>[2x]MALTKLVDAGAWQVEVAPAGTVQDSLVFLSPRNFGGVPGTGVDSVAAIEAALAAGDVDLGGEHWFISRPIYCVSGRTIQNGKISTLAAQGSGFMAGSIFAPGNYHPVYVDPVPKLACSSTNGSATITVSSHEFVVGDLVRLSSTRGIIGSDAVLVPWYMQLARVVGVSGDTVKLDAPIDTTETLVVHKATPAGYNARFNKPLFVLERATFRNIEVDTWDYWTADSATFECAFEGIRGKARSVVYGNTFCRTNFDNIDITFSNKASEMAFGSHDTNLSNIKFRADSQNWDSTNSVGISWAESGRRCTLDNWQLLVPQGVNLSVLVRISSHRDVQIRKGFIQVHSSSNNILSVEHYGGDRPPCNNILFEDIDVNATGAAAVVVDVYKSANDSAINAVRFEGISYRGATPSVALMRQRGTTSNQVTGVRASLYSANGGAFLVSSAMAWDVRLYGPGLQVPAAVAVLGRTAVLSASRSNLHALRWVTEAIIGVTSTTPGNVLREAVIPAGTLRASDYIDFVISGSTGGATSTKDVLVGVLDSGSNFQGVGFTAPTTEESYYTVQGRISFPTTGNCLITATIGRAGVGVSYARTLVSISNYTTNDVKLQVQAWVGSSAGSLSVQHGCFAPSELTGKGHHHHHH

Virion-associated depolymerases are large trimeric and multi-domain proteins that constitute the phage arsenal to degrade the polysaccharide layers in their bacterial host. In this study, we elucidated the structural and functional features of the capsular depolymerase KP34gp57 from the Klebsiella phage KP34. The CPS depolymerase KP34gp57 is a large enzyme with a trimeric organization consisting of 630 amino acid residues per chain and an MW of the trimer of ~200 kDa. In this work, we focused on the structure and function of the CPS depolymerase KP34gp57 derived from Klebsiella phage KP34, which efficiently causes a visible halo zone on bacterial lawns of the K63 serotype of K. pneumoniae.

Surprisingly, we collected diffraction data at 2.0 Å resolution, which produced a unit cell and space group (a = 38.3, b = 141.0, c = 81.9; β = 102.6, space group P21) not compatible with the size of the protein. Therefore, it appeared obvious that KP34gp57 had encountered some proteolytic degradation prior to crystallization. Only upon experimental structure determination using SAD did electron density maps clearly reveal two copies of the portion 27–454 in the unit cell, i.e., missing the C-terminal domain. The N-terminal region of each copy (residues 27–56) contains two α-helices, followed by the typical β-helix structure characterizing the catalytic domain of tailspikes (residues 57–102 and 204–454). In addition, a six-stranded β-barrel domain protrudes from the catalytic β-helix between residues 103–203. This crystal structure content was fully unexpected since monomeric tailspikes have hitherto never been observed and their trimeric state is believed to be crucial for enzyme stability. Indeed, we identified a large cavity in each promoter (with an area of 280.9 Å2 and a volume of 330.5 Å3), formed by both the β-helix and the β-barrel insertion domain, using the software CASTp. A clear electron density describes the catalytic pocket, thus allowing for the identification of E266 and E300 (belonging to the β-helix structure) as the most promising catalytic residues and D151 (belonging to the insertion domain) as likely assisting CPS binding. After incubation of CPS with the enzyme variants, the absorption of all samples was analyzed at 490 nm and compared with a calibration curve measured with known concentrations of glucose. This assay confirmed the crucial role of E266 and E300 in catalysis since E266Q/E300Q is fully inactive. In KP34gp57, the high resistance of this CBM to proteolysis, together with the observation of the monomeric state of KP34gp57 once deprived of the CBM, suggests that the CBM domain plays a crucial role in inducing a compact trimerization of the enzyme while still allowing for the necessary flexibility needed by the catalytic domain for enzymatic catalysis.(4aS,5aR)-N-{1-[(R)-[(2R)-1,1-dioxidotetrahydro-2H-thiopyran-2-yl](phenyl)methyl]-1H-pyrazol-4-yl}-5,5-difluoro-5a-methyl-1,4,4a,5,5a,6-hexahydrocyclopropa[f]indazole-3-carboxamide | C25 H27 F2 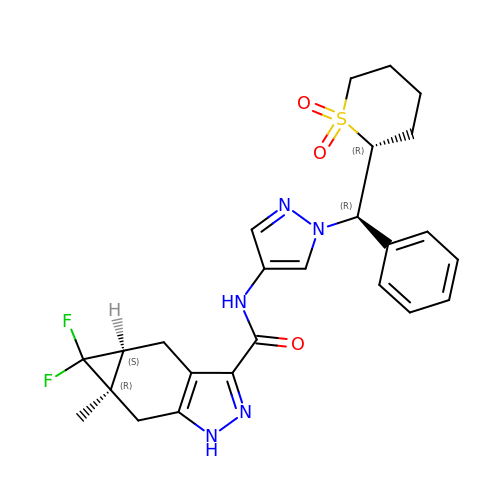N5 O3 S | JNRFIKALOWSUBG-DAVFGYKESA-N>[2x]ASAWPEEKNYHQPAILNSSALRQIAEGTSISEMWQNDLQPLLIERYPGSPGSYAARQHIMQRIQRLQADWVLEIDTFLSQTPYGYRSFSNIISTLNPTAKRHLVLACHYDSKYFSHWNNRVFVGATDSAVPCAMMLELARALDKKLLSLKTVSDSKPDLSLQLIFFDGEEAFLHWSPQDSLYGSRHLAAKMAST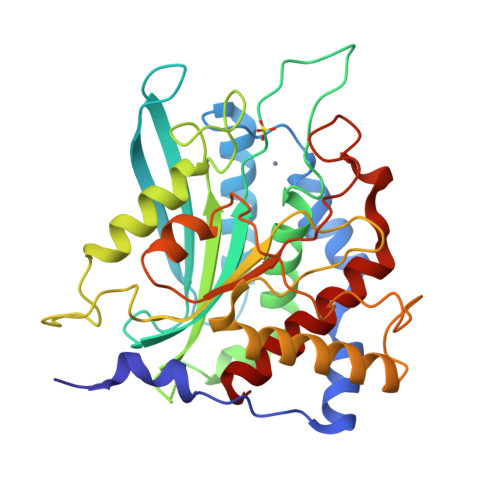PHPPGARGTSQLHGMDLLVLLALIGAPNPTFPNFFPNSARWFERLQAIEHELHELGLLKDHSLEGRYFQNYSYGGVIQDDHIPFLRRGVPVLHLIPSPFPEVWHTMDDNEENLDESTIDNLNKILQVFVLEYLHL>MNKKRLLLLSVFLVSVFVPVLVADVIYYYQGQITVGNVAPPMYFAIQPNGNAKIGNNSNVPSYINAQPSSGGSGFTAQVNITNATYNYYFNFMGLAVSKTGYIYLAKVAYSYTATNNPIQNATLYIMNQQGQIVYKYKLIVNGVVNSTLPSTPLQINSGSYIVSLLIVPYQGTLPKTPSNDLATITVNFGFSPMTASPPPIPLPSP[9x]

The model archaeaon Sulfolobus acidocaldarius assembles three filaments of the type-IV pilus superfamily (archaella, archaeal adhesion pili and UV-inducible pili), as well as a so-far uncharacterised fourth filament, named “thread”. The filament is highly glycosylated and consists of subunits of the protein Saci_0406, arranged in a head-to-tail manner. Saci_0406 displays structural similarity, but low sequence homology, to bacterial type-I pilins. Thread subunits are interconnected via donor strand complementation, a feature reminiscent of bacterial chaperone-usher pili.

Applying these values to the 3D refinement resulted in a map of 4.02 Å resolution, which further improved to 3.45 Å after several rounds of CTF refinement. Our atomic model reveals that each subunit consists of an N-terminal β-strand (tail) followed by a globular (head) domain. The head domain contains two β- sheets composed of 11 β-strands. On the subunit level, one β-strand is missing to complete the sheet, leaving a gap between β-4 and β-12. Upon closer investigation of the assembled filament, this missing strand is replaced by the β1 tail strand of the next subunit along the filament (n+1). In the thread, the β-tail from subunit n, extends further into the subunit two positions along the filament (n − 2). β;− 1 of the subunit n is partially buried in the subunits n − 1 and n − 2, further adding to the stability of the interaction. Threads appear to be covalently interlinked by a non-canonical isopeptide bond between Asn57 of subunit n and the N-terminal Asp24 of the subunit n + 2. Along the map of the S. acidocaldarius thread, we found dead-end protrusions that did not resemble the protein backbone or side chains. These protrusions were exclusively found at asparagine residues N56, N80, N83, N121 and N146 of each thread subunit. Connected to each of the five glycosylation sites at the corresponding asparagine are two N-acetylglucosamine (GlcNAc) residues, the second of which branches to bind two individual Mannose (Man), Glucose and one 6-sulfoquinovose molecule. Whereas the threads have a rise of 31.6 Å and twist of –103.2°, Type I pili have a reported rise of 7.7 Å and a twist of 115°.4-[[[4-[(4-chlorophenyl)methyl-cyclopentyl-sulfamoyl]phenyl]sulfonyl-(piperidin-4-ylmethyl)amino]methyl]-2-(methylamino)benzoic 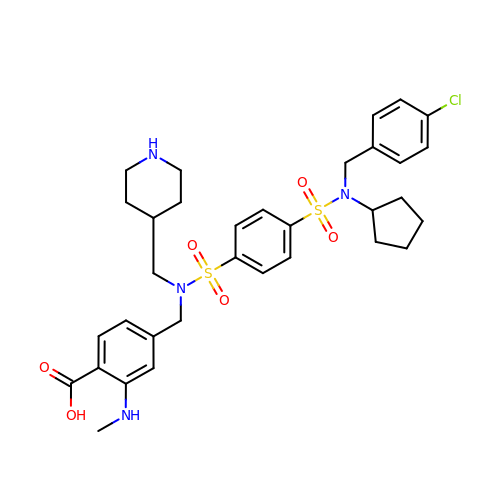acid | C33 H41 Cl N4 O6 S2 | AAUHXDBDDJEFRE-UHFFFAOYSA-N>MAKNRRDRNSWGGFSEKTYEWSSEEEEPVKKAGPVQVLIVKDDHSFELDETALNRILLSEAVRDKEVVAVSVAGAFRKGKSFLMDFMLRYMYNQESVDWVGDYNEPLTGFSWRGGSERETTGIQIWSEIFLINKPDGKKVAVLLMDTQGTSDSQSTLRDSATVFALSTMISSIQVYNLSQNVQEDDLQHLQLFTEYGRLAMEETFLKPFQSLIFLVRDWSFPYEFSYGADGGAKFLEKRLKVSGNQHEELQNVRKHIHSCFTNISCFLLPHPGLKVATNPNFDGKLKEIDDEFIKNLKILIPWLLSPESLDIKEINGNKITCRGLVEYFKAYIKIYQGEELPHPKSM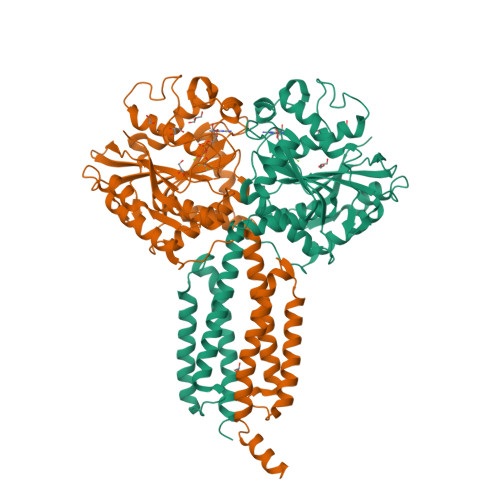LQATAEANNLAAVATAKDTYNKKMEEICGGDKPFLAPNDLQTKHLQLKEESVKLFRGVKKMGGEEFSRRYLQQLESEIDELYIQYIKHNDSKNIFHAARAAALEHHHHHH[2x]> VSEIKTLVTFFGGTGDLAKRKLYPSVFNLYKKGYLQKHFAIVGTARQALNDDEFKQLVRDSIKDFTDDQAQAEAFIEHFSYRAHDVTDAASYAVLKEAIEEAADKFDIDGNRIFYMSVAPRFFGTIAKYLKSEGLLADTGYNRLMIEKPFGTSYDTAAELQNDLENAFDDNQLFRIDHYLGKEMVQNIAALRFGNPIFDAAWNKDYIKNVQVTLCEVLGVEERAGYYDTAGALLDMIQNHTMQIVGWLAMEKPESFTDKDIRAAKNAAFNALKIYDEAEVNKYFVRAQYGAGDSADFKPYLEELDVPADSKNNTFIAGELQFDLPRWEGVPFYVRSGKRLAAKQTRVDIVFKAGTFNFGSEQEAQEAVLSII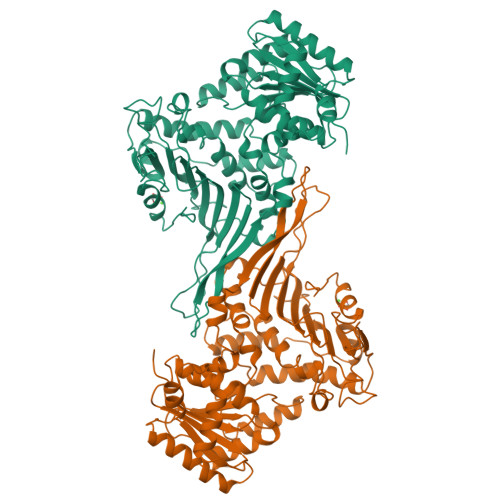IDPKGAIELKLNAKSVEDAFNTRTIDLGWTVSDEDKKNTPEPYERMIHDTMNGDGSNFADWNGVSIAWKFVDAISAVYTADKAPLETYKSGSMGPEASDKLLAANGDAWVFKG> MLFYSFFKTLIDTEVTVELKNDMSIRGIL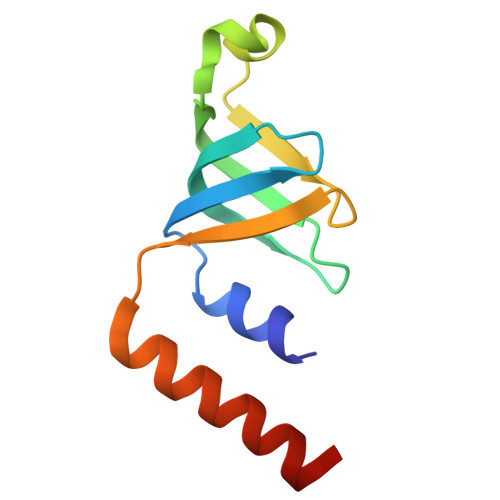KSVDQFLNVKLENISVVDASKYPHMAAVKDLFIRGSVVRYVHMSSAYVDTILLADACRRDLANNKRQ>[2x]GSHMSENFAVATPVRVGIVGTGYAAQRRAEVFRGDRRSQLVSFWGNSEANTAKFADTFGVRPQQSWQALINDPEIDLVLIATINQLHGAIAEAALQAGKHVVLEYPLALTYAMGKKLQQLAREKGKLLHVEHIELLGGVHQAIRQNLGKIGEVFYARYSTIMGQNPAPQRWTYHHQQFGFPLVAALSRISRFTDLFGTVQQVDAQCRFWDQPN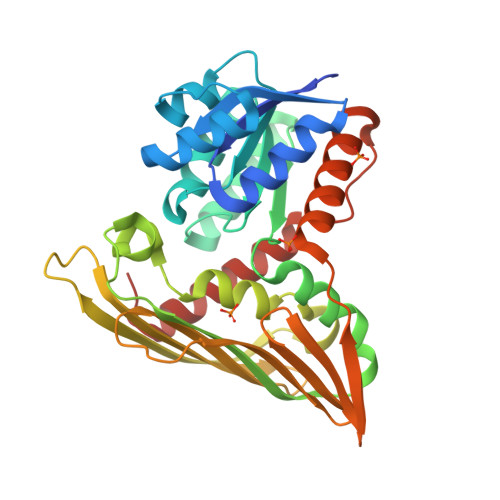PEYFRACLATAYLQFNNGLKAEVIYGKGEVFHQNERIFTLHGDRGTLIFVGETGRLIQGQTETEITVGSRRGLFRQDTEAVLDYLTTGKPLYVDLEASLYALEVADLCAQACGYKVEN> GPGKGKKLNEASRQQRFNTSIRDFEFWLSEAETLL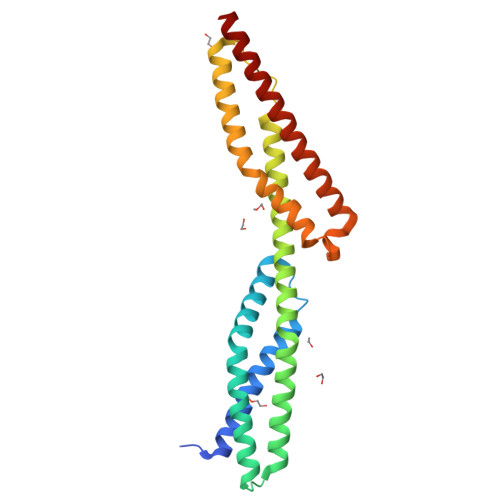AMKDQARDLASAGNLLKKHQLLEREMLAREDALKDLNTLAEDLLSSGTFNVDQIVKKKDNVNKRFLNVQELAAAHHEKLKEAYALFQFFQDLDDEESWIEEKLIRVSSQDYGRDLQGVQNLLKKHKRLEGELVAHEPAIQNVLDMAEKLKDKAAVGQEEIQLRLAQFVEHWEKLKELAKARGLKLEESLEYLQFMQ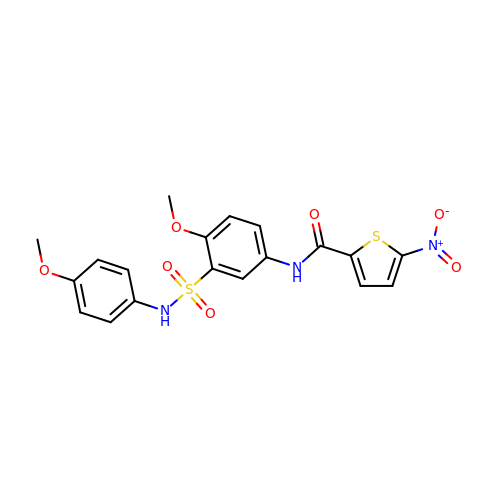N-{4-methoxy-3-[(4-methoxyphenyl)sulfamoyl]phenyl}-5-nitrothiophene-2-carboxamide | C19 H17 N3 O7 S2 | DYOXCKGIGMXWNR-UHFFFAOYSA-N>MPYVEIIEQPKQRGMRFRYKCEGRSAGSIPGERSTDTTKTHPTIKINGYTGPGTVRISLVTKDPPHRPHPHELVGKDCRDGYYEADLCPDRSIHSFQNLGIQCVKKRDLEQAISQRIQTNNNPFHVPIEEQRGD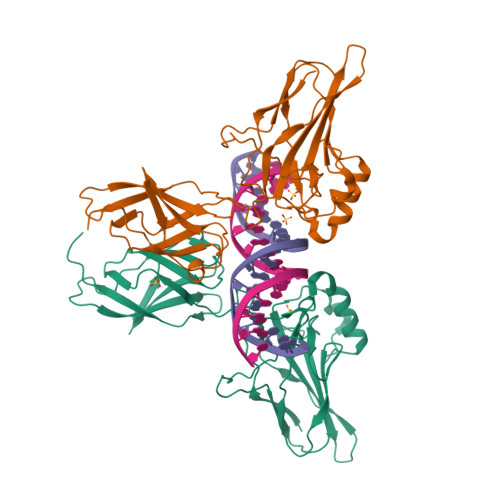YDLNAVRLCFQVTVRDPAGRPLLLTPVLSHPIFDNRAPNTAELKICRVNRNSGSCLGGDEIFLLCDKVQKEDIEVYFTGPGWEARGSFSQADVHRQVAIVFRTPPYADPSLQAPVRVSMQLRRPSDRELSEPMEFQYLPDTDDRHRIEEKRKR[2x]> MTNNSERKRLEKRIAQLCKFIGRSPWVFHVNSGSCNGCDIEIIAALTPRYDAERFGVKLVGSPRHADILLVTGPVTNQSLERVKLVYEQTPDPKIVIAIGACPTGGSVFYESPFTNAPLDRIIPVDVFVPGCPPRPEAILHGVVLALEKLAKMIKGEVPPEEGEE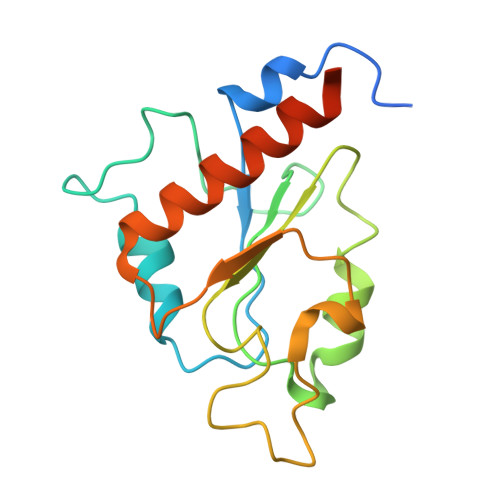NE>[2x]MRILAIDTATEACSVALWNNGTINAHFELCPREHTQRILPMVQEILAASGASLNEIDALAFGRGPGSFTGVRIGIGIAQGLALGANLPMIGVSTLATMAQGAWRKTGATRVLAAIDARMGEVYWAEYQRDAQGVWQGEETEAVLKPERVGERLKQLSGEWATVGTGWSAWPDLAKECGLTLHDGEVSLPAAEDMLPIASQKLAAGETVAVEHAEPVYLRNEVAWKKLPGKE;>[2x]MRVLGIETSCDETGIAIYDDKKGLLANQLYSQVKLHADYGGVVPELASRDHV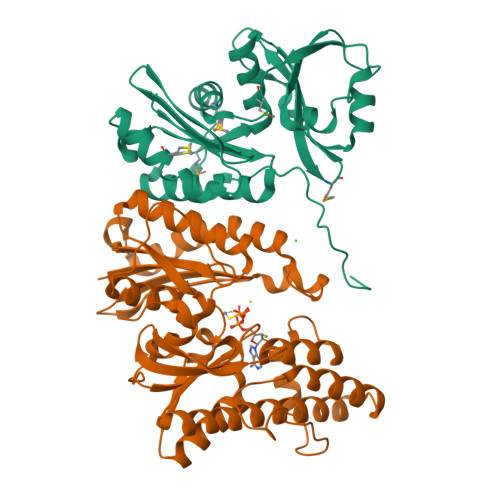RKTVPLIQAALKEAGLTASDIDAVAYTAGPGLVGALLVGATVGRSLAFAWNVPAIPVHHMEGHLLAPMLEDNPPEFPFVALLVSGGHTQLISVTGIGQYELLGESIDDAAGEAFDKTAKLLGLDYPGGPMLSKMASQGTAGRFVFPRPMTDRPGLDFSFSGLKTFAANTIRSNGGDEQTRADIARAFEDAVVDTLMIKCKRALESTGFKRLVMAGGVSANRTLRAKLAEMMQKRRGEVFYARPEFCTDNGAMIAYAGMVRFKAGVTADLGVTVRPRWPLAELPAA> MSPNNQNEYEIIDATPSTSVSNDSNRYPFANEPTNALQNMDYKDYLKMSAGNVSEYPGSPEVFLSEQDAVKAAIDIVGKLLTGLGVPFVGPIVSLYTQLIDILWPSKQKSQWEIFMEQVEELINQKIAEYARNKALSELEGLGNNYQLYLTALEEWKENPNGSRALRDVRNRFEILDSLFTQYMPSFRVTNFEVPFLTVYTMAANLHLLLLRDASIFGEEWGLSTSTINNYYNRQMKLTAEYSDHCVKWYETGLAKLKGSSAKQWIDYNQFRREMTLTVLDVVALFSNYDTRTYPLATTAQLTREVYTDPLGAVDVPNIGSWYDKAPSFSEIEKAAIRPPHEFDYITGLTVYTKKRSFTSDRYMRYWAGHQISYKTIGTSSTFTQMYGTNQNLQSTSNFDFTNYDIYKTLSNDAVLLDIVYPGYTYTFFGMPETEFFMVNQLNNTRKTLTYKPASKDIIDRTRDSELELPPETSGQPNYESYSHRLGHITFIYSSSTSTYVPVFSWTHRSADLTNTVKSGEITQIPGGKSSYIGRNTYIIKGRGYTGGDLLALTDRIGSCEFQMIFPESQRFRIRIRYASNETSYISLYGLNQSGTLKFNQTYSNKNENDLTYNDFKYIEYPRVISVNASSNIQRLSIGIQTNTNLFILDRIEFIPVDETYEAETDLEAAKKAVNALFTNTKDGLQPGVTDYEVNQAANLVECLSDDLYPNEKRLLFDAVREAKRLSEARNLLQDPDFQ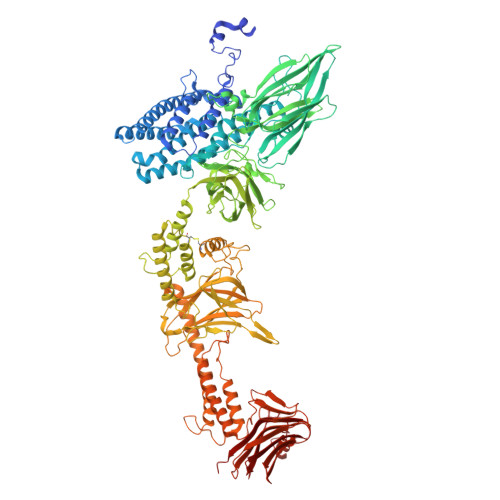EINGENGWTASTGIEVIEGDAVFKGRYLRLPGAREIDTETYPTYLYQKVEEGVLKPYTRYRLRGFVGSSQGLEIYTIRHQTNRIVKNVPDDLLPDVPPVNNDGRINRCSEQKYVNSRLEVENRSGEAHEFSIPIDTGELDYNENAGIWVGFKITDPEGYATLGNLELVEEGPLSGDALERLQKEEQQWKIQMTRRREETDRRYMASKQAVDRLYADYQDQQLNPNVEITDLTAAQDLIQSIPYVYNEMFPEIPGMNYTKFTELTDRLQQAWGLYDQRNAIPNGDYRNELSNWNTTSGVNVQQINHTSVLVIPNWNEQVSQKFTVQPNQRYVLRVTARKEGVGNGYVSIRDGGNQSETLTFSASDYDTNGMYDTQASNTNGYNTNSVYNDQTGYITKTVTFIPYTNQMWIEISETEGTFYIESVELIVDVE> VEPSVQVGYSPEGSARVLVLSAIDSAKTSIRMMAYSFTAPDIMKALVAAKKRGVDVKIVIDERGNTGRASIAAMNYIAN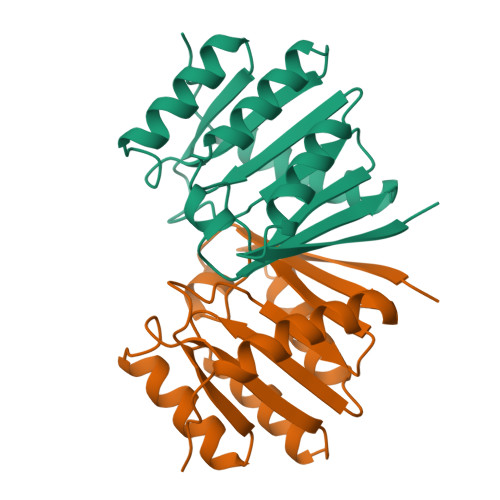SGIPLRTDSNFPIQHDKVIIVDNVTVETGSFNFTKAAETKNSENAVVIWNMPKLAESFLEHWQDRWNQGRDYRSSY>MASMREDYSLECDPAVIGTAVKGKEAVHSDLGYWIESEKNDTWRLKRAHLIEMKTCEWPKSHTLWTDGIEESDLIIPKSLAGPLSHHNTREGYRTQMKGPWHSEELEIRFEECPGTKVHVEETCGTRGPSLRSTTASGRVIEEWCCRECTMPPLSFRAKDGCWYGMEIRPRKEPESNLVRSMVTA[2x]

The flavivirus NS1 is a ~48 kDa conserved non-structural protein with two conserved N-linked glycosylation sites and six intra-molecular disulfide bonds. NS1 consists of the N-terminal β-roll, the middle wing, and the C-terminal β-ladder domains. Two NS1s are assembled into a symmetric, head-to-head dimer through domain swapping of the β-rolls and the extension of β-sheets from the β-ladders. Although not being a component of the virion, NS1 represents a marker for host immune recognition and evasion.

To understand the function of ZIKV NS1, we solved the crystal structure of ZIKV NS1172–352 from ZIKV strain Suriname (KU312312). The crystal of ZIKV NS1 β-ladder domain (NS1172–352) diffracted to a 2.8 Å resolution in Fourier space. Two β-ladder protomers were found in each asymmetric unit. These two protomers form a symmetric, head-to-head dimer through an extended, 14-stranded β-sheet seen in the dimeric assembly of DENV and WNV NS1 β-ladder structures. The dimer interface buries a total surface area of 1628 Å2. In ZIKV NS1, K227 forms a salt bridge with D234, while H253 interacts with W232 through a π-π stacking interaction at physiological pH. Remarkably, T233A, one of the mutations found in the Natal_RGN strain (KU527068), which was isolated from fetal brain tissue with severe microcephaly, is located at the NS1 dimer interface. The hydroxyl group of T233 is central in organizing a hydrogen-bonding network across the dimer interface. In particular, it has been shown that T233 also plays a pivotal role in organizing a hydrogen-bonding network across the dimer interface in other solved ZIKV NS1 structures. These structural data suggests that mutation of Thr233 to Ala would disrupt this elaborated network, and could potentially impair the stability of the dimer. Over 49% of T233A mutant are in the monomeric state. This percentile is much higher than that of the parent Suriname NS1 β-ladder domain, suggesting that T233A mutation interferes the self-association of ZIKV NS1 β-ladder domain.>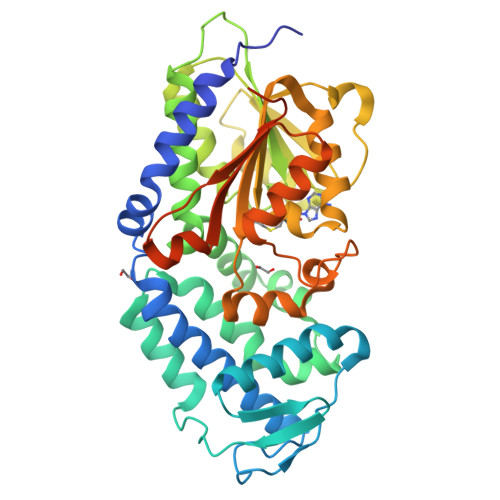 MVLFPELGGSILPKSAILDAFRIAKEATDDFILNGQLGTYYNEVMPRSTELCVAHIVNAFEQLGCPIRSAAAYQRLERVPYLPKHERFMNLIYGLLEEARLIDINGSEITRTSVPVSTKSVETMLEELLHDEPLHAAEHKLTSLTGSKFADCITGKEDGLQLIFGSPEGREIVTDVYAKSPINAVWIQQAEFFLEQLVKRLPNTGEPLRILEMGAGTGGTTVKMLPLLERLGVPVEYTMTDLSSSLIAAARKRFKKYPFMKFKVVNIESPPDPQLVHSQHIILATNCVHATRNLEISTRNIHRILRPDGFLLLLEMTEQVPWVDFIFGLLEGWWLFEDGRRHALQPATHWKKILTSVGYGHVDWTEGTRPEANIQRLIIALASEPRYDHTPQSLQPPVQVPLTDAALEHHHHHH>MGSDKIHHHHHHENLYFQGMGIRHIALFRWNDTVTPDQVEQVITALSKLPAAIPELKNYAFGADLGLAAGNYDFAVVADLD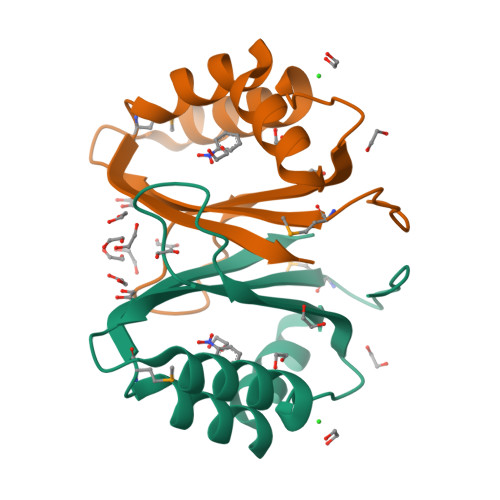GEDGFRAYQDHPDHRAALAIIAPMLADRVAVQFAL[2x]> MTGTMKIYYEHDADLGFILGKKVAVLGFGSQGHAHAHNLKDSGVDVRVGLRKGSRSWEKAEAAGLRVLPVAEAVREADVVMVLLPDEKQAQVYREEVEPNL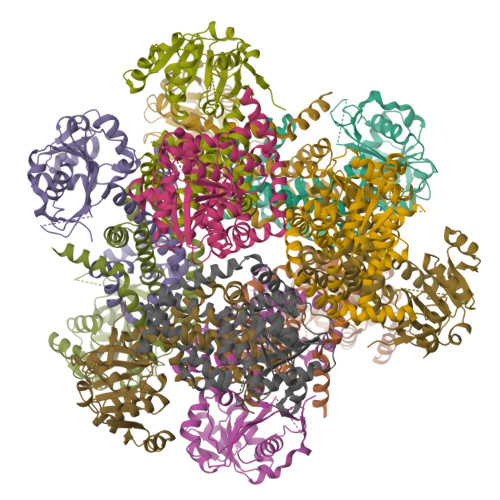KEGGALAFAHGFNVHFGQIKPRKDLDVWMVAPKGPGHLVRSEYGGGSNWSHPQFEKRPPGGSGVPALVAVHQDASGSAFPTALAYAKAIGAARAGVIATTFKDETETDLFGEQAVLCGGLTRLIRAGFETLVEAGYPPEMAYFETVHEVKLIVDLIYEAGLKGMRYSISNTAEYGDYTRGDLAVPLEETKRRMREILRQIQSGEFAREWMLENQVGSPVLEANRKRWAAHPIEEVGSRLRAMMRS> GSTKPFGVNRGLDLDKILHCYQMNDDLFMFV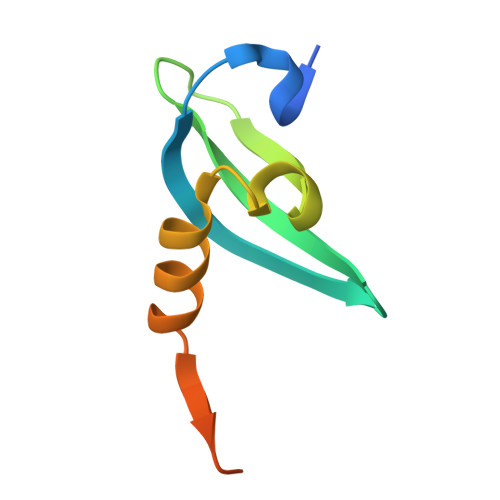TWKGCSSIDAVHINDIKEAYPLQIIKYFESLRIIVPKGSGSGSGSGS> MIHEVDEVLKALLKGGALTDSGIDVAFEAPTRDWAARRNAPVVNAYLYDIREDVGRRHRGQVAVRDQDDIVVKRRQPPRWFRLSYLVTAWTKTPQDEHRLLSAVLATLLPREQLPPYELPGALGAMNLPVPMTVAGVQTESRSLAEI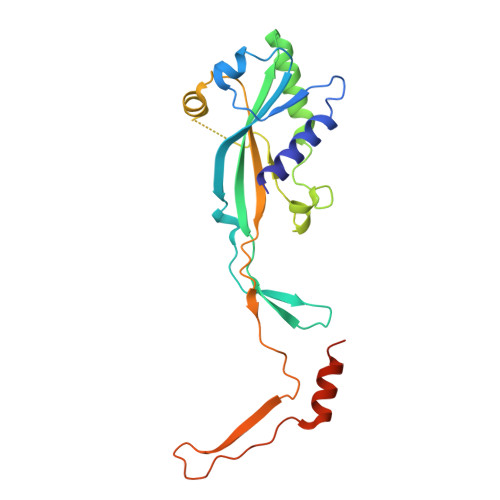WSALGGELKPSLDLVVTAPFPAYPEYDAGPPVTEGATVRIGGVEGDPPMSEGRSHRPHQVAAARAARKAVTDGRTKRQ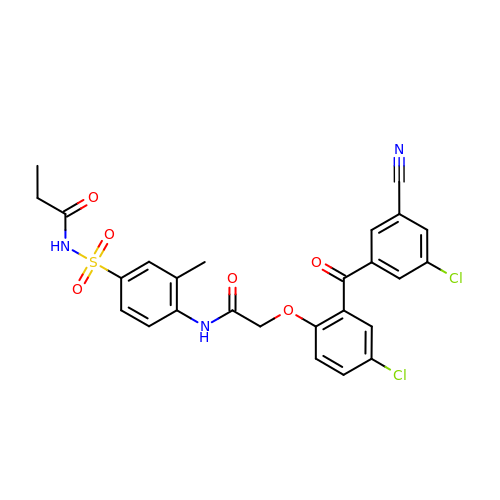N-({4-[({4-chloro-2-[(3-chloro-5-cyanophenyl)carbonyl]phenoxy}acetyl)amino]-3-methylphenyl}sulfonyl)propanamide | C26 H21 Cl2 N3 O6 S | GAQZNFUDILDDDI-UHFFFAOYSA-N>AASMAQRMVWVDLEMTGLDIEKDQIIEMACLITDSDLNILAEGPNLIIKQPDELLDSMSDWCKEHHGKSGLTKAVKESTITLQQAEYEFLSFVRQQTPPGLCPLAGNSVHEDKKFLDKYMPQFMKHLHYRIIDVSTVKELCRRWYPEEYEFAPKKAASHRALDAISESIKELQFYRNNIFK[2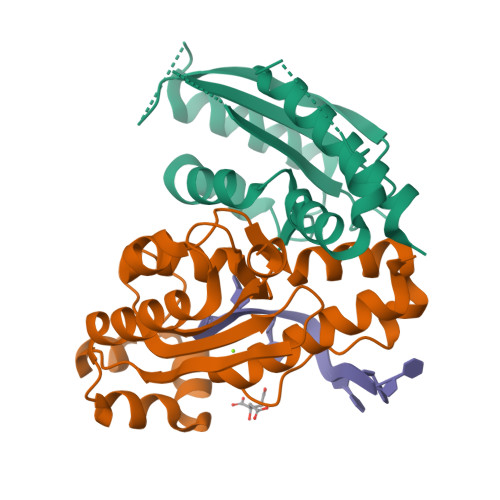x]>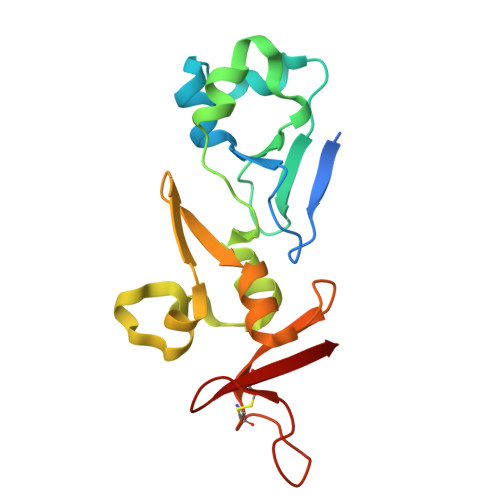[2x]MGSSHHHHHHSSMKSLILPPNEFLDHYILNAEFHRFAGISKNAYKFWKNVEIGRYQGTRIIFLHRNCILEKHQQALRQCSGLNGFVLASAFCSFTGLAPSHLVEKNNSSIYKLLELKEICGIKFVNLKKFYDFLGLNYHQHIYIEKCHFFSPAPFEKRIKITESMCVGYY>PMILGYWDIRGLAHAIRLLLEYTDSSYEEKKYTMGDAPDYDRSQWLNEKFKLGLDFPNLPYLIDGAHKITQSNAILCYIARKHNLCGETEEEKIRVDILENQTMDNHMQLGMICYNPEFEKLKPKYLEELPEKLKLYSEFLGKRPWFAGNKITFVDFLVYDVLDLHRIFEPKCLDAFPNLKDFISRFEGLEK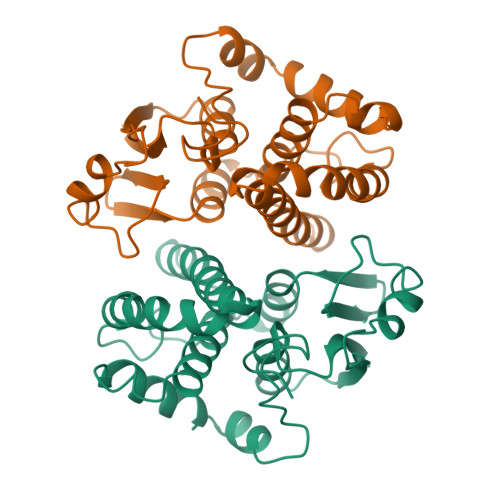ISAYMKSSRFLPRPVFSKMAVWGNK[4x]N-(carboxycarbonyl)-S-(3-nitrobenzyl)-L-cysteine 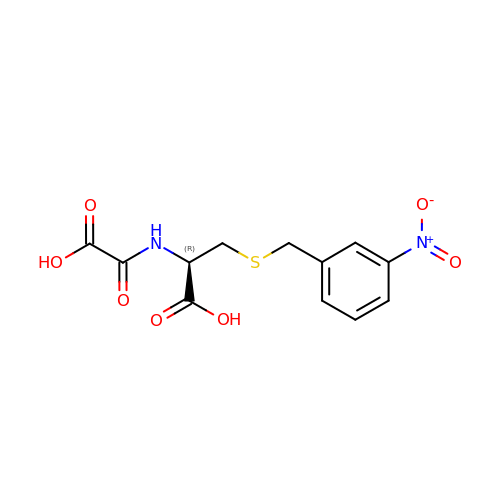| C12 H12 N2 O7 S | OBSYIMVMIJBTMQ-VIFPVBQESA-N>[2x]MLKILWTYILFLLFISASARAEKPWYFDAIGLTETTMSLTDKNTPVVVSVVDSGVAFIGGLSDSEFAKFSFTQDGSPFPVKKSEALYIHGTAMASLIASRYGIYGVYPHALISSRRVIPDGVQDSWIRAIESIMSNVFLAPGEEKIINISGGQKGVASASVWTELLSRMGRNNDRLIVAAVGNDGADIRKLSAQQRIWPAAYHPVSSVNKKQDPVIRVAALAQYRKGETPVLHGGGITGSRF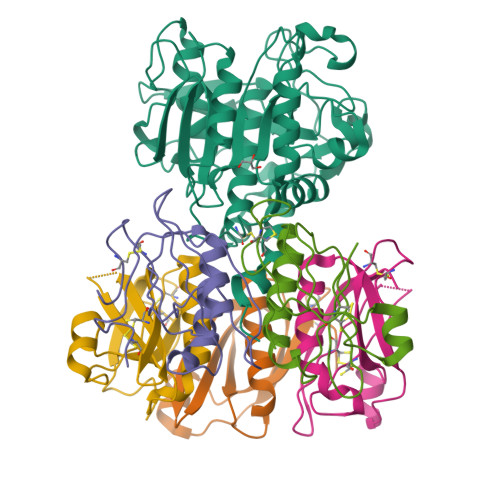GNNWVDIAAPGQNITFLRPDAKTGTGSGTSEATAIVSGVLAAMTSCNPRATATELKRTLLESADKYPSLVDKVTEGRVLNAEKAISMFCKKNYIPVRQGRMSEEL;>[10x]EWTGDARDGMFSGVVITQFHTGQIDNKPYFCIEGKQSAGSSISACSMKNSSVWGASFSTLYNQALYFYTTGQPVRIYYEPGVWTYPPFVKALTSNALVGLSTCTTSTECFGPDRKKNSLE>MSSLLQQTSQLLVQSYQSDNIAFKSTKQFPEKKSFLELELIQKILFPDFFTRRDKRTFNNVLERLSLLVYHIQNSIEAYYNQQLAEKCITALLSQFVTIRELVKQDIIAAYTGDPAASSLAMIIRSYPGIHVMMIQRVAHILYMNGDIEYSRELMENIHSVTG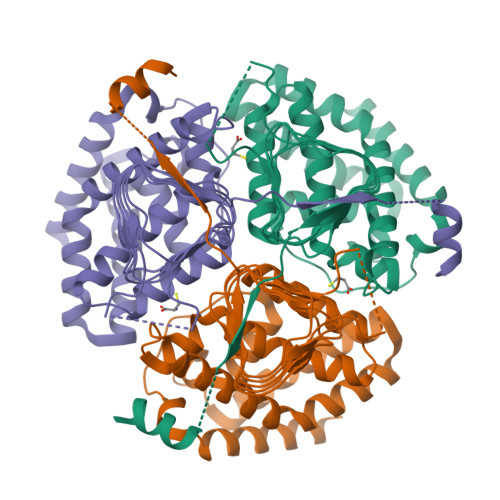IDIHPGTSIGNHFFIDHGVGVVIGETAVIGNWCRVYQSVTLGAMSFKEDNGIVIKGNKRHPTIGDFVVIGAGAKVLGNITIGSNVKIGANCWITQNIDQDQIVFISEHPSQITKSSTKQSSKDDKIILQSLTENKISEEQENLSWVNSPELLCTYTSEESTPINLDCFVSCQQ[3x]>[2x]MRYRLAWLLHPALPSTFRSVLGARLPPPERLCGFQKKTYSKMNNPAIKRIGNHITKSPEDKREYRGLELANGIKVLLISDPTTDKSSAALDVHIGSLSDPPNIAGLSHFLEHMLFLGTKKYPKENEYSQFLSEHAGSSNAFTSGEHTNYYFDVSHEHLEGALDRFAQFFLSPLFDESAKDREVNAVDSEHEKNVMNDAWRLFQLEKATG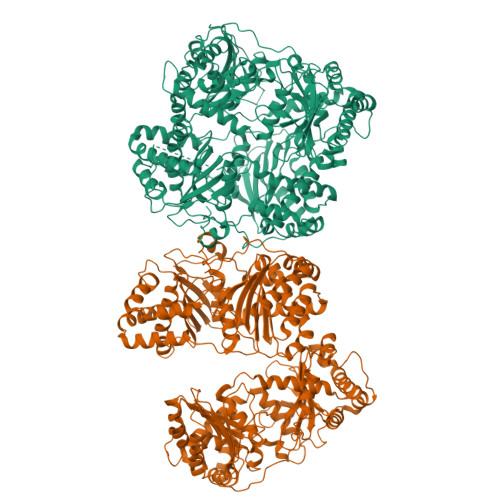NPKHPFSKFGTGNKYTLETRPNQEGIDVRQELLKFHSAYYSSNLMAVVVLGRESLDDLTNLVVKLFSEVENKNVPLPEFPEHPFQEEHLKQLYKIVPIKDIRNLYVTFPIPDLQKYYKSNPGHYLGHLIGHEGPGSLLSELKSKGWVNTLVGGQKEGARGFMFFIINVDLTEEGLLHVEDIILHMFQYIQKLRAEGPQEWVFQELKDLNAVAFRFKDKERPRGYTSKIAGILHYYPLEEVLTAEYLLEEFRPDLIEMVLDKLRPENVRVAIVSKSFEGKTDRTEEWYGTQYKQEAIPDEVIKKWQNADLNGKFKLPTKNEFIPTNFEILPLEKEATPYPALIKDTAMSKLWFKQDDKFFLPKANLNFEFFSPFAYVDPLHSNMAYLYLELLKDSLNEYAYAAELAGLSYDLQNTIYGMYLSVKGYNDKQPILLKKIIEKMATFEIDEKRFEIIKEAYMRSLNNFRAEQPHQHAMYYLRLLMTEVAWTKDELKEALDDVTLPRLKAFIPQLLSRLHIEALLHGNITKQAALGIMQMVEDTLIEHAHTKPLLPSQLVRYREVQLPDRGWFVYQQRNEVHNNSGIEIYYQTDMQSTSENMFLELFAQIISEPAFNTLRTKEQLGYIVFSGPRRANGIQGLRFIIQSEKPPHYLESRVEAFLITMEKSIEDMTEEAFQKHIQALAIRRLDKPKKLSAESAKYWGEIISQQYNFDRDNTEVAYLKTLTKEDIIKFYKEMLAVDAPRRHKVSVHVLAREMDSSPVVGEFPSQNDINLSQAPALPQPEVIQNMTEFKRGLPLFPLVKPH>QGNDTSEVMLLDTGWEFSQSGTEKWMPATVPGTVHQDLISHELLPNPFYGMNEKKIQWVENEDWEYRTSFIVSEEQLNRDGIQLIFEGLDTYADVYLNGSLLLKADNMFVGYTLPVKSVLRKGENHLYIYFHSPIRQTLPQYASNGFNYPADNDHHEKHLSVFSRKAPYSYGWDWGIRMVTSGVWRPVTLRFYDIATISDYYVRQLSLTDENARLSNELIVNQIVPQKIPAEVRVNVSLNGTTVTEVKQQVTLQPGINHITLPAEVTNPVRWMPNGWGTPTLYDFSAQIACGDRIVAEQSHRIGLRTIRVVNEKDKDGESFYFEVNGIPMFAKGANYIPQDALLPNVTTERYQTLFRDMKEANMNMVRIWGGGTYENNLFYDLADENGILVWQDFMFACTPYPSDPTFLKRVEAEAVYNIRRLRNHASLAMWCGNNEILEALKYWGFEKKFTPEVYQGLMHGYDKLFRELLPSTVKEFDSDRFYVHSSPYLANWGRPESWGTGDSHNWGVWYGKKPFESLDTDLPRFMSEFGFQSFPEMKTIAAFAAPEDYQIESEVMNAHQKSSIGNSLIRTYMERDYIIPESFEDFVYVGLVLQGQGMRHGLEAHRRNRPYCMGTLYWQLNDSWPVVSWSSIDYYGNWKALHYQAKRAFAPVLINPIQQNDSLSVYLISDRLDTMEQMTLEMKVVDFDGKTLGKKIQVHSLEVPANTSKCVYRAKLDGWLTPEDCRRSFLKLILKDKSGHQVAESVHFFRKTK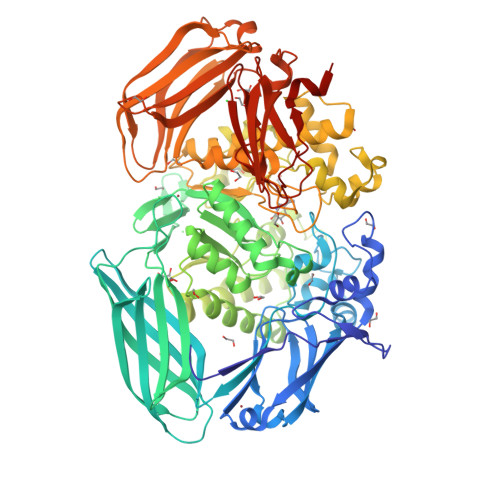DLQLPPTSVSYQMKQTDGKCELTLFSSMLAKDIFIETPLQGARYSDNFFDLLPGERKKVIITSPRIKKGEELPVNIKHIRETYKEHHHHHH[2x]> GHMPSSGK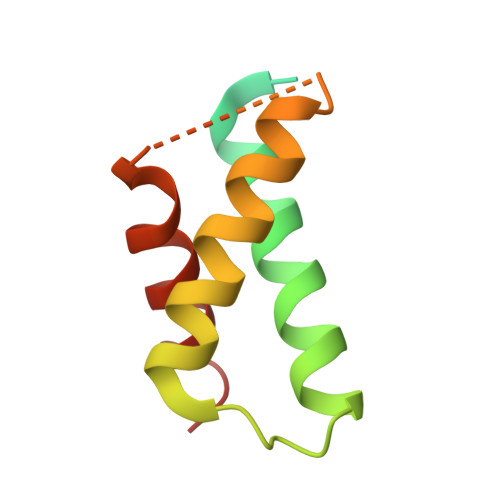RRAPRRVYQIPQRRRLQGKDPRWATMADLKMQAVKEICYEVALADFRHGRAEIEALAALKMRELCRTYGKPDGPGDAWRAVARDVWDTVGE> IIGGRESRPHSRPYMAYLQIQSPAGQSRCGGFLVREDFVLTAAHCWGSNINVTLGAHNIQRRENTQQHITARRAIRHPQYNQRTIQNDI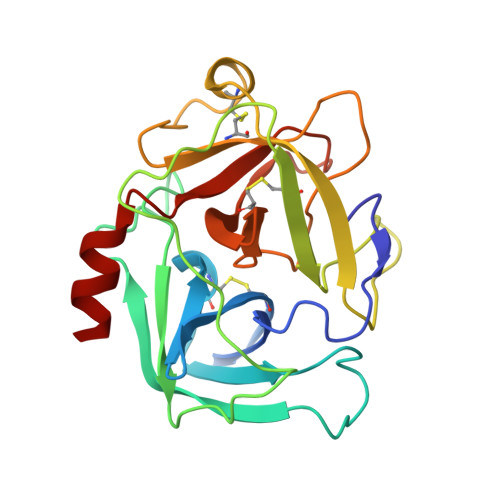MLLQLSRRVRRNRNVNPVALPRAQEGLRPGTLCTVAGWGRVSMRRGTDTLREVQLRVQRDRQCLRIFGSYDPRRQICVGDRRERKAAFKGDSGGPLLCNNVAHGIVSYGKSSGVPPEVFTRVSSFLPWIRTTMR Alongshan virus (ALSV), a newly discovered member of unclassified Flaviviridae family, is able to infect humans. ALSV NSP1 is a typical flavivirus NS5-like protein. It carries two essential enzymatic activities: the methyltransferase (MTase) and the RNA-dependent RNA polymerase (RdRp). The flaviviral NS5-MTase functions to catalyze the methylation of viral RNA cap.

The crystals of ALSV MTase bound with SAM and SAH were individually obtained by co-crystallization at a protein/ligand molar ratio of 1:3. The structure of ALSV MTase in complex with SAH was solved at 2.1 Å, with Rwork and Rfree values of 0.210 and 0.236, respectively. In each case, clear electron densities for the bound ligands were observed, which enabled us to define, at the atomic level, the SAM/SAH-binding pocket. In the complex structures, the SAM/SAH molecule fits into a conserved pocket located at the edge of the ALSV MTase core region. The pocket is surrounded by helices αX, αA and αD, strands β1-β4, and several adjacent loops. The SAM/SAH molecule lies down in the pocket, within which the bound ligand is stabilized by multiple hydrogen-bond interactions. These include residues S99, G129, W130 and D183 of the MTase forming five hydrogen bonds with the methionine/homocysteine group of SAM/SAH, and amino acids L148, N168 and V169 mediating another three hydrogen bonds with the adenosyl group of SAM/SAH. For ALSV MTase, the binding affinities of SAM and SAH to the refolded enzyme were determined to be 8.1 ± 3.3 μM and 4.1 ± 1.8 μM, respectively. In ALSV MTase, this loop is of short length and high flexibility, devoid of any stabilizing contacts with the SAM/SAH ligand. SAM/SAH binds to ALSV MTase in a 1:1 molar ratio and 2. the SAM/SAH-binding pocket in ALSV MTase is largely unoccupied during expression.

>[4x]GPLGSEVYKGDGYKVWKLEPSLGDPLELGRKTKTEMNAMTHDEFDRMKYRGVVAEVYSGDKPSKGYDKLRVLLDLMDRPRLGTTVDLCAGRGGWSELVKDLEGPKGITAVSLWERGKEEWMADPAIHRINANVKHLRPWQVDTLLFDGGEAFKRDQNLRKEENFNDSLLDAVDAWMMQPVPPRNFVIKIQVPYTQKAIALLEKWQVKTGKGRLVRLAGDRLSNTVMYFLSVRLETQIRGRVTTFVRELAERRKDRSLTADPSLQYERVEPQWTEEAR> GSQQRKVLTLEKG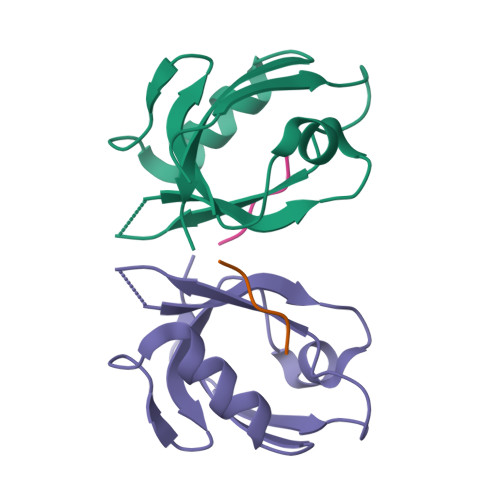DNQTFGFEIQTYGLHHREEQRVEMVTFVARVHESSPAQLAGLTPGDTIASVNGLNVEGIRHREIVDIIKASGNVLRLETLYGT;> SSSSL> PISPIETVPVKLKPGMDGPKVKQWPLTEEKIKALVEICTEMEKEGKISKIGPENPYNTPVFAIKKKDSTKWRKLVDFRELNKRTQDFWEVQLGIPHPAGLKKNKSVTVLDVGDAYFSVPLDEDF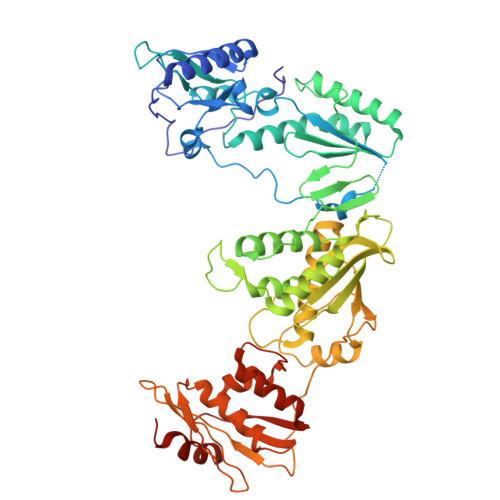RKYTAFTIPSINNETPGIRYQYNVLPQGWKGSPAIFQSSMTKILEPFKKQNPDIVIYQYMDDLYVGSDLEIGQHRTKIEELRQHLLRWGLTTPDKKHQKEPPFLWMGYELHPDKWTVQPIVLPEKDSWTVNDIQKLVGKLNWASQIYPGIKVRQLCKLLRGTKALTEVIPLTEEAELELAENREILKEPVHGVYYDPSKDLIAEIQKQGQGQWTYQIYQEPFKNLKTGKYARMRGAHTNDVKQLTEAVQKITTESIVIWGKTPKFKLPIQKETWETWWTEYWQATWIPEWEFVNTPPLVKLWYQLEKEPIVGAETFYVDGAANRETKLGKAGYVTNKGRQKVVPLTNTTNQKTQLQAIYLALQDSGLEVNIVTDSQYALGIIQAQPDKSESELVNQIIEQLIKKEKVYLAWVPAHKGIGGNEQVDKLVSAGIRKIL> RMVDLPVLQPRLCTHARWPAPIYGLLVDPSLPSNPQWQNGRVHVDGTLLGTTPVSGSWVSCFAAEAAYEFQSGTGEVATFTLIEQDGSAYVPGDRAAPLGYPDFSGQL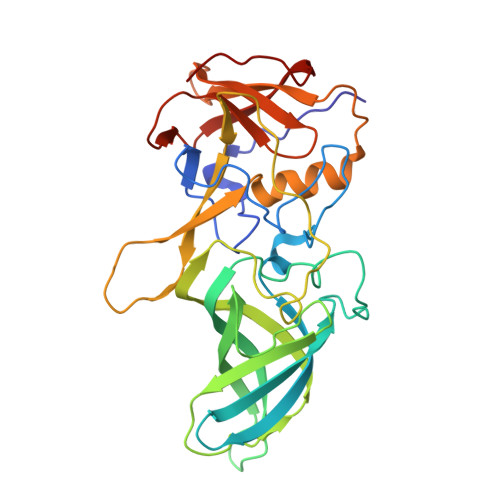EIEVQTETTKTGDKLKVTTFEMILGPTTNVDQAPYQGRVYASLTAVASLDLVDGRVRAVPRSIYGFQDVIPEYNDGLLVPLAPPIGPFLPGEVLLRFRTYMRQLDTADAAAEAIDCALPQEFISWFASNAFTVQSDALLLRYRNTLTGQLLFECKLYSEGYIALSYSGSGPLTFPTDGFFEVVSWVPRLFQLASV>CSAMGTAIKKRNLEVKTQMSETIWLEPSNNKTVYLQIKNTSDKDMSGLQAKIASAVTSKGYQVVSNPDTAGYWIQANVLKADKMDLRESQGWLSRGYEGAVTGAALGAGITAYNSSSAGATLGVGLAAGLVGMAADAMVEDVNYTMITDVQIAERTKTQVQTDNVAVLRQGTSGTKVQTSTETGNQHKYQTRVVSNANKVNLKFPEAQPVLEDQLAKSIANILGSG[10x]

Following transfer of IncF-like plasmids, recipients become refractory to a second wave of conjugation with the same plasmid via entry (TraS) and surface (TraT) exclusion mechanisms. SFX, which is mediated by the OMP TraT, is specific for Gram-negative bacteria. TraT is a highly expressed ~24 kDa lipoprotein with a copy number of approximately 29,000–84,000 copies/cell. In this work, we determined the cryo-EM structure of TraT encoded by pKpQIL (TraTpKpQIL) and the F (TraTF) plasmid derivative, pOX38, at 2.47 Å and 2.66 Å resolution respectively. This revealed that lipidated TraT oligomerises into a decameric champagne cork-like structure, composing of a transmembrane α-helical barrel domain and an extracellular ring domain.

To gain insights into the molecular mechanism of SFX, we purified recombinant TraTpKpQIL from E. coli OM vesicles in CYMAL-6 and determined the cryo-EM structure. Analysis of the purified TraTpKpQIL by mass spectrometry confirmed that the first cysteine of the mature protein (C36) is modified by DAG and PA, which agrees with previous reports. The map displays 10-fold symmetry corresponding to ten copies of TraTpKpQIL. Each TraTpKpQIL protomer consists of three amphipathic TM helices (α1, α3 and α4) that anchors it to the OM, a central β-sandwich domain (β1–β7) that is flanked by two α-helices (α2 and α5) that protrudes to the extracellular space; β5 and β6 form a β-hairpin perpendicular to the top of the β-sandwich domain. Each protomer associates with one DAG molecule, where interactions occur exclusively between DAG and its own protomer. DAG is found in the interface of the TM helices α1, α3 and α4 and forms a hydrogen bond between its diacylglycerol moiety and the backbone of T137. The decameric structure is predominately stabilised by interactions between the extracellular domain of the protomers; the α-helical barrel domain does not display significant interactions with adjacent protomers. The arrangement between the β-sandwich domains, including the β5 and β6 intertwining, results in the formation of a cyclic architecture that consists of an inner β-barrel with a diameter of 48 Å. The conjugation frequency of pKpQIL into recipients expressing TraTpKpQIL was reduced by a log-fold, −3.6, compared to the baseline level of conjugation, −2.5, in the absence of TraTpKpQIL.>MRTTKFLALALCLLASASALSANNSAPSNDWWDIPYPSQFDVKSLKTQSFISVKGNKFIDDKGKTFTFRGVNIADTGKLLSRNQWQKSLFEELANNWGVNTIRLPIHPVSWRKLGPDVYLGHIDEAVRWANDLGIYLILDWHSIGYLPTEQYQHPMYDTTIKETRDFWRRITFRYQNVPTVAVYELFNEPTTMGNTLGERNWAEWKTLNESLIDMIYASDKTVIPLVAGFNWAYDLSPIKKAPIEREGIAYAAHPYPQKAKPEVKNDKNFFKLWDEKWGFAADTYPVIATQLGWVQPDGYGAHIPV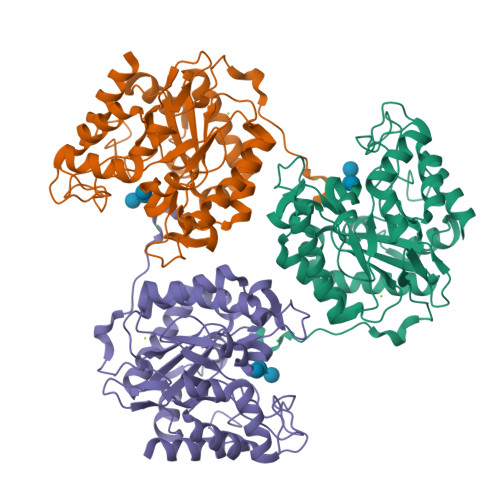KDDGSYGPRIVKYMQKKGVSYTVWVFDPDWSPTMINDWDFTPSEQGAFFKQVMLEAKKR[6x]> YEANYEDVIKKYKPADAKLDRIAYDWRLHGGVTPV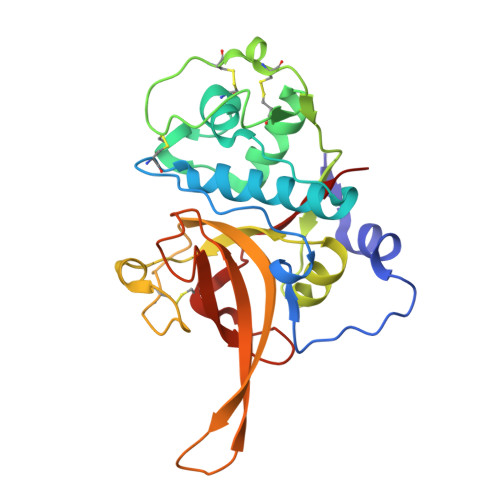KDQALCGSCWAFSSVGSVESQYAIRKKALFLFSEQELVDCSVKNNGCYGGYITNAFDDMIDLGGLCSQDDYPYVSNLPETCNLKRCNERYTIKSYVSIPDDKFKEALRYLGPISISIAASDDFAFYRGGFYDGECGAAPNHAVILVGYGMKDIYNEDTGRMEKFYYYIIKNSWGSDWGEGGYINLETDENGYKKTCSIGTEAYVPLLE> EEPVPVPTEQTVFMYLPWSDNLTSNFYQNISDLESVVEKNILKDERIIIFMCTTATKATLFELAYENGKSVHKTLKNYTDPAYTTAEGITSILNDVQRYSPTKRYSMVIGCHGMGWIPVSNSKSRSGLRTKMHWEYENVPMTR;> YFGGLNAQYQTDITTLAKGISNAGLKMEYILFDDCYMSSIEVAYALKDVTDYLIGSTSEVMAYGMPYAEIGQYLIGKVDYAGICDGFYSFYSTYSTPCGTIAVTDCSELDNLATIMKEINHRY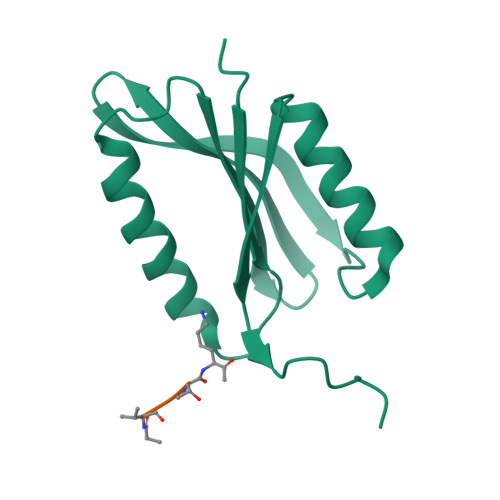TFDPSLTSSLQRLDGYYPVIFFDYGDYVSKLCPDETLVARFNEQLNRTVPFKRNTEYFYSMSRGEVKINTFSGITISDPSTHSLASKKEETAWYAATHLEHHHHHH> AANRAPTSVNAQEVHRWLQSFNWDFKNNRTKYATKYKMANETKEQFKLIAKEYARMEAVKDERQFGSLQVALTRLNAGVRVHPKWNETMKVVSNFLEVGEYNAIAATGMLWDSAQAAEQKNGYLAQVLDEIRHTHQCAYVNYYFAKNGQDPAGHNDARRTRTIGPLWKGMKRVFSDGFISGDAVECSLNLQLVGEACFTNPLIVAVTEWAAANGDEITPTVFLSIETDELRHMANGYQTVVSIANDPASAKYLNTDLNNAFWTQQKYFTPVLGMLFEYGSKFKVEPWVKTWDRWVYEDWGGIWIGRLGKYGVESPRSL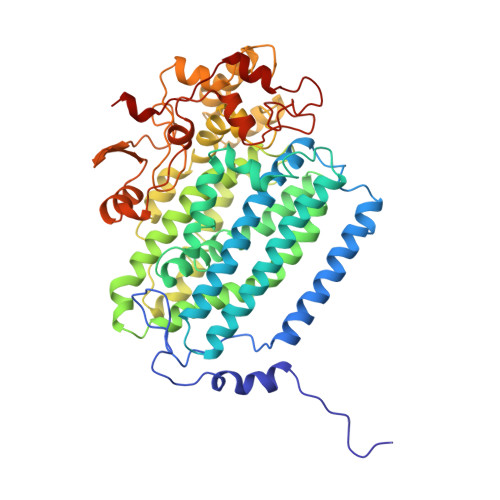KDAKQDAYWAHHDLYLLAYALWPTGFFRLALPDQEEMEWFEANYPGWYDHYGKIYEEWRARGCEDPSSGFIPLMWFIENNHPIYIDRVSQVPFCPSLAKGASTLRVHEYNGEMHTFSDQWGERMWLAEPERYECQNIFEQYEGRELSEVIAELHGLRSDGKTLIAQPHVRGDKLWTLDDIKRLNCVFKNPVKAF>[2x]HHHHHHSSGLVPRGSHMNAADESLGNVLLVGLGAVAIQVALDLRRHGAGRLGALNHPGRRSQRIAEALARGACLQLEGQGQHRWLSGNAALDVFHQDPAELRDDWQTLVLCVPADSYLDVVRGLPWERLGGVRTLLLVSAFIGA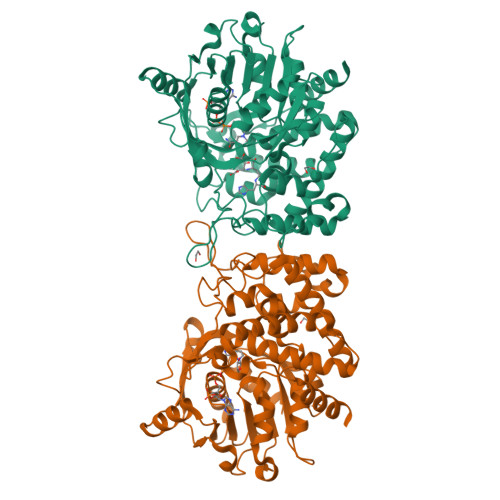NLLVRSALPAGCQATVLSLSSYYAATKVIDETQPLRALTKAVKRRVYLGSSRPDCPARETWRRVLAGSGVEVVPLATPEAAEGRNVTTYVHSPFFLGEFALARILSEQGPPGFMYKLYPEGPITPGAIGAMRRLWCELSELLRRMGAEPLNLLRFLNDDNYPVHETMLPRASIDGFAEAGAERQEYLLFVRYAALLVDPFSPADEQGRHFDFSAVPFRRVSRDEDGLWRLPRVPLEDYRKLALIVALAAHFDLAMPQARSLLASYENAVSRFIDCQGASQCHPSLYPIDSRPAADAIYRQWCSTC> GPHMTRIIYDRKFLMECRNSPVT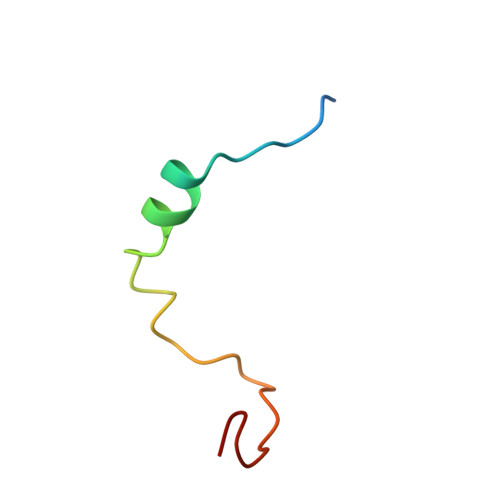KTPPRDLPTIPGVTS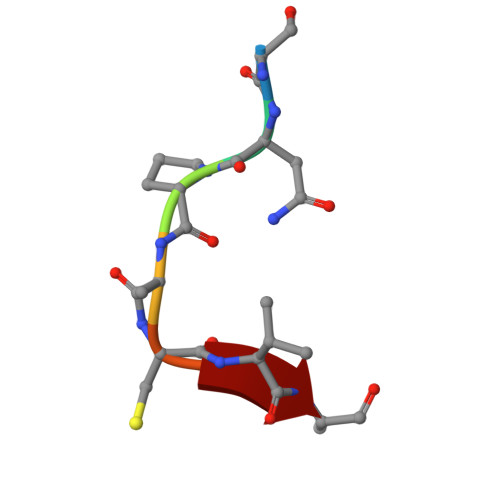> SNPACVA>[4x]MDYCNKKHTAEEYVKISDNNYVPFPEAFSDGGITWQLLHSSPETSSWTAIFNCPAGSSFASHIHAGPGEYFLTKGKMEVRGGEQEGGSTAYAPSYGFESSGAL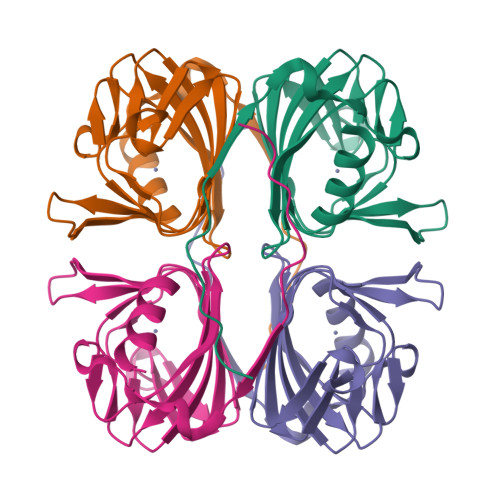HGKTFFPVESQFYMTFLGPLNFIDDNGKVIASIGWAEAQGAWLATKNEAA>[2x]MAEIPKEMLRAQTNVI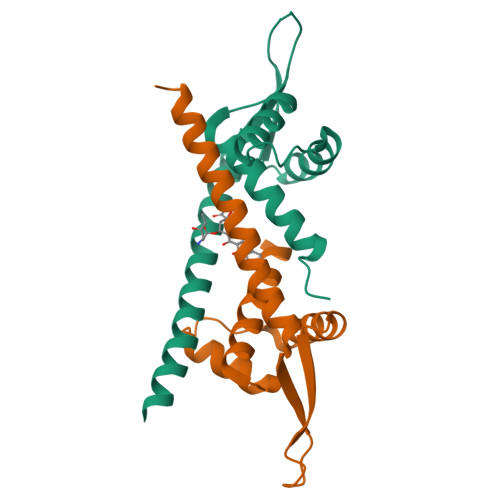LLNVLKQGDNYVYGIIKQVKEASNGEMELNEATLYTIFKRLEKDGIISSYWGDESQGGRRKYYRLTEIGHENMRLAFESWSRVDKIIENLEANKKSEAIKSRWSHPQFEK> MPWDFNNYYSHNMDGLISKLKLSKTESDKLKALRQIVRERTRDVFQEARQVAIDVRRQALTLESVRLKLEKTNVRYLSPEERADLARLIFEMEDEARDDFIKFQPRFWTQGSFQYDTLNRPFHPGQEMDIDDGTYMPMTVFESEPSIGHTLLLLLVDTSLKSLEAENDGWVFEEKNTCGRIKIYREKTHIDVPMYAIPKEQFQKKQTAADSAHLIKSDSVFESFALNRGGREAYAVESDKVNLALREGVRRWSVSDPKIVEDWFNESCKRIGGHLRSVCRFMKAWRDAQWEVGGPSSISLMTAVVNILDRES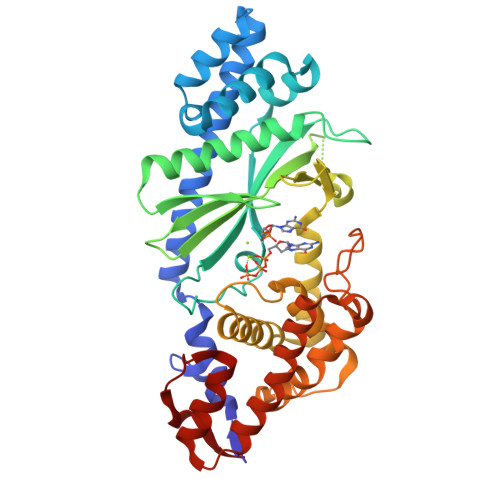HNGSDLTGTMKLIARLLPEEFNRGVESPDDTDEKPLFPAESNHNVHHRAIVETMEGLYGILLAAEQSESREEALRKINEAFGKRVTNALLITSSA> SMIKSYAAKEAGGELEVYEYDPGELRPQDVEVQVDYCGICHSDLSMIDNEWGFSQYPLVAGHEVIGRVVALGSAAQDKGLQVGQRVGIGWTARSCGHCDACISGNQINCEQGAVPTIMNRGGFAEKLRADWQWVIPLPENIDIESAGPLLCGGITVFKPLLMHHITATSRVGVIGIGGLGHIAIKLLHAMGCEVTAFSSNPAKEQEVLAMGADKVVNSRDPQALKALAGQFDLIINTVNVSLDWQPYFEALTYGGNFHTVGAVLTPLSVPAFTLIAGDRSVSG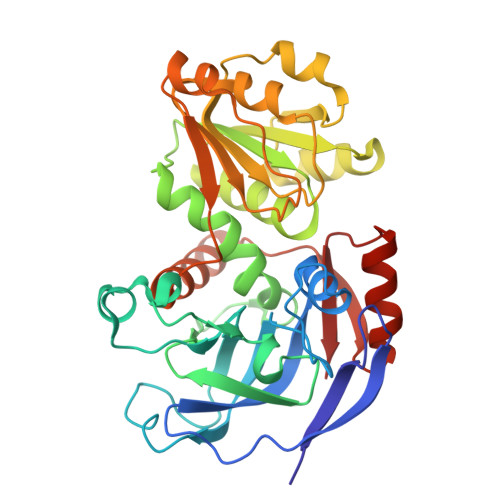SATGTPYELRKLMRFAARSKVAPTTELFPMSKINDAIQHVRDGKARYRVVLKA>GPNSGTLALLLDEGSKQLPQAIIIGVKKGGTRALLEFLRVHPDVRAVGAEPHFFDRSYDKGLAWYRDLMPRTLDGQITMEKTPSYFVTREAPARISAMSKDTKLIVVVRDPVTRAISDYTQTLSKRPDIPTFES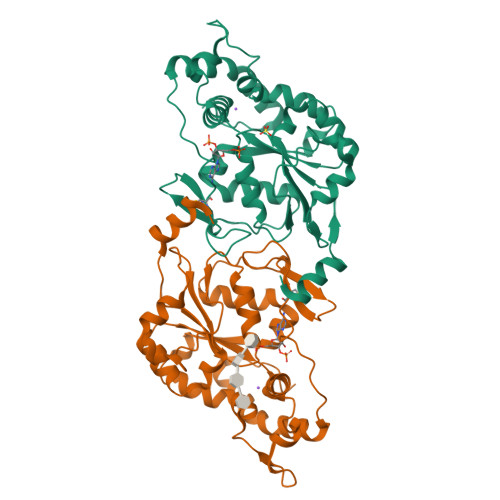LTFKNRTAGLIDTSWSAIQIGIYAKHLEHWLRHFPIRQMLFVSGERLISDPAGELGRVQDFLGLKRIITDKHFYFNKTKGFPCLKKAEGSSRPHCLGKTKGRTHPEIDREVVRRLREFYRPFNLKFYQMTGHDFGWDG[2x]In contrast, modification of cytoplasmic proteins with a single O-linked N-acetylglucosamine (O-GlcNAc)4 is a regulatory post-translational modification that is dependent on a single O-GlcNAc-transferase (OGT), which transfers the O-GlcNAc moiety onto target proteins, and O-GlcNAcase (OGA), which can reverse this process. In this report, we describe the identification of the first complete putative bacterial protein O-GlcNAcylation system, found in the soil thermophile Thermobaculum terrenum. We identified the products of genes Tter_2822 (hereafter Ttogt) and Tter_0116 (hereafter Ttoga) as putative OGT and OGA orthologues, respectively. To investigate the catalytic machinery and conservation of substrate/product binding modes, we determined the crystal structures of TtOGT and TtOGA.

TtOGT was co-crystallized with the product of O-GlcNAc transfer, UDP. The structure, solved by molecular replacement and refined against synchrotron diffraction data of 2.8 Å, revealed an ordered N-terminal TPR domain and a bilobal catalytic domain at the C terminus. The TtOGT TPR domain itself displays good structural similarity with that of hOGT (r.m.s.d. = 1.3 Å for 106 Cα atoms). However, a deletion at the region previously designated as the tetratricopeptide-like region (TLR) results in a major change in the orientation of the TPR domain relative to the GT41 catalytic domain compared with hOGT. This more direct/rigid fusion of the TtOGT TPRs to the GT41 domain compared with that of hOGT creates a relatively narrow groove for the protein substrates to bind near the active site. However, the GT41 domain of TtOGT is similar to that of hOGT (r.m.s.d. = 1.5 Å for 303 Cα atoms) despite the absence of the intervening domain of unknown function that is positioned between the two lobes of this domain in hOGT. Catalysis of O-GlcNAc transfer is facilitated by the pro-RP oxygen of the α-phosphate acting as the catalytic base. It is proposed that the presence of an oxyanion hole formed by backbone amides of His920, Thr921, and Thr922 (equivalent to Cys422, Thr423, and Thr424 in TtOGT; maximum atomic shift of 1.7 Å), an α-helical electrostatic dipole, and the evolutionarily conserved Lys842 (Lys341in TtOGT) function together to ensure the correct positioning of the donor substrate and to stabilize the negative charge developing on the leaving group. Strikingly, the hydrophobic pocket formed by Met501, Leu502, and Cys917 at the hOGT active site, which fits the N-acetyl moiety of UDP-GlcNAc in the hOGT active site, is not apparent in the TtOGT·UDP complex. It is possible that a conformational change is required to form this hydrophobic pocket and perhaps to reorient the TPRs to create an active site groove that is more permissive for docking of a protein substrate.

>MTTRDAATIKALLSHAHEAQRSGDVLASERACWRVLQIAPDNSEALHLLGLLHGECGNYGLAATLLRRAVALDPGEASYHYNLGNVLVASGQVERGITSLHHALELRPDYHRAHSGLYVALHYSALYDPRARHILALDWARRYADPLTPVPATPVDPDPHRRLRIGYVSGELRCHPVGYFLEPVIEAHDRTAYEVYCYSNDPRSDALTDRLRALSDRWRDVWPLTDAELCELVRRDGIDILVDLSWHLGMHRLFAFARRPAPVQVTWLAAINTTGMRAMDYLVGDQHLCPPGSDELYTERLVRLSRFYLPCNPPPDLPGWAPADPLGRGFPVFGCFNRLSMIGPEVLDLWAKILLALPRARLRLIATGLQDPVTSSRLMRALEGRGVAGERLELLSPMPRTDLLATYNDIDVALDTLPYSGCTTSLEALWMGVPVVTLEGADMAGRATSSLLRWAGLQELVSRTQEEYIDIALGLGRDLGTLARLREHLRRWLRSVSMSDQGSFTAELEDAYRRMWRDACQTAAGRQGA[4x]(4aS,7S)-4a-methyl-7-(prop-1-en-2-yl)-2,3,4,4a,5,6,7,8-octahydroquinolinium | C13 H22 N 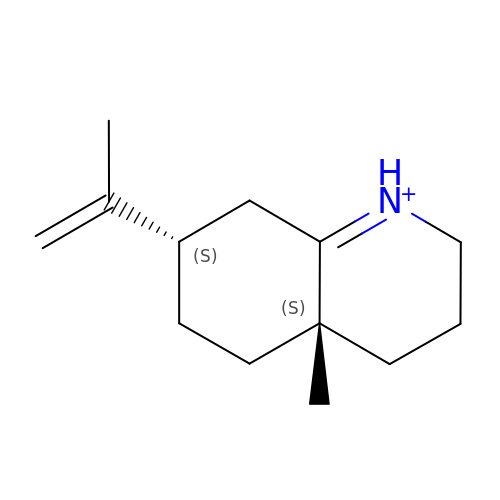| IUOUFRPMLZKTGM-WCQYABFASA-O1-[(1R)-1-(2-fluorophenyl)ethyl]piperazine | C12 H17 F N2 | 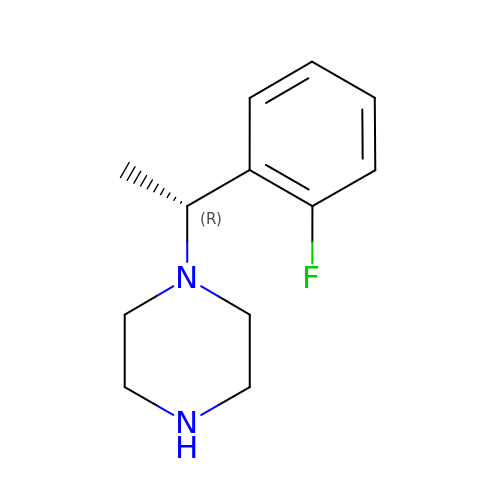UIJNEACQJVSKLI-SNVBAGLBSA-N> MSKNRSSLQSGPLNSELLEEQKQEIYEAFSLFDMNNDGFLDYHELKVAMKALGFELPKREILDLIDEYDSEGRHLMKYDDFYIVMGEKILKRDPLDEIKRAFQLFDDDHTGKISIKNLRRVAKELGETLT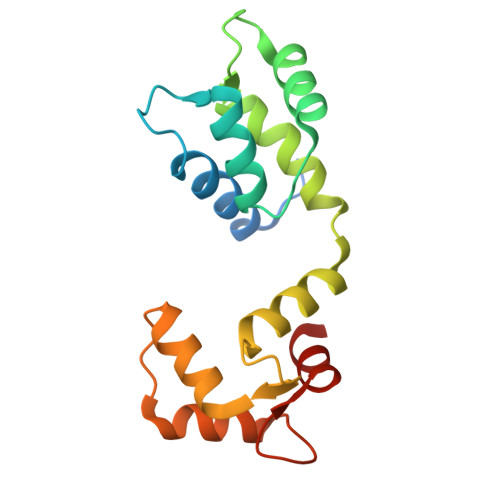DEELRAMIEEFDLDGDGEINENEFIAICTDS>MDFVSGDKDTTSVTVESKDNGKRTEVKIGAKTSVIKDHNGKLFTGKELKDANNNGVTVTETDGKDEGNGLVTAKAVIDAVNKAGWRVKTTGANGQNDDFATVASGTNVTFADGNGTTAEVTKANDGSITVKYNVKVADGLKLDLEHHHHHH[9x]

The Haemophilus surface fibril (Hsf) is an unusually large trimeric autotransporter adhesin (TAA) expressed by the most virulent strains of H. influenzae. Hsf is known to mediate adhesion between pathogen and host, allowing the establishment of potentially deadly diseases such as epiglottitis, meningitis and pneumonia. TAAs, which are part of the type V family of secreted proteins, have three major types of domains arranged in a linear fibril ‘lollipop’ structure. The two binding domains of Hia (HiaBD1 and HiaBD2) have also been identified in Hsf; unlike Hia, however, Hsf has an additional binding domain (HsfBD3) and three putative domains, the structure and function of which are unknown.

In our effort to characterize the full-length Hsf protein, we determined the crystal structure of trimeric PD1 at a resolution of 3.3 Å, thus providing the first insight into the molecular arrangement of Hsf to date. HsfPD1 crystallized in the monoclinic space group C2, with nine monomers in the asymmetric unit. The individual monomers of HsfPD1 are comprised of three distinct domains that fold to form well characterized TAA domains. The N-terminus of HsfPD1 spans 29 amino acids participating in the unexpected formation of three β-sheets, βW11, βW12 and βW13 (where ‘W’ represents tryptophan), which share considerable structural homology with the C-terminal TrpRing domain. The KG domain is composed of two β-strands, βKG1 and βKG2, as well as three α-helices, αKG1, αKG2 and αKG3. The C-terminal TrpRing is composed of five β-strands: βW21, βW22, βW23, βW24 and βW25. All domains participate in extensive intertwining, where the C-terminal α-helices (αKG3) from each monomer come together to create the central core of the trimer interface. Since our construct contained only 29 N-terminal residues upstream of the KG domain, and as TrpRing domains typically consist of ∼55 amino acids, the structural evidence suggests that our N-terminal β-strands constitute the latter half of a TrpRing domain.>[6x]NSVGQGEFGGAPFKRFLRGTRIVSGGKLKRMTREKAKQVTVAGVPMPRDAEPRHLLVNGATGTGKSVLLRELAYTGLLRGDRMVIVDPNGDMLSKFGRDKDIILNPYDQRTKGWSFFNEIRNDYDWQRYALSVVPRGKTDEAEEWASYGRLLLRETAKKLALIGTPSMRELFHWTTIATFDDLRGFLEGTLAESLFAGSNEASKALTSARFVLSDKLPEHVTMPDGDFSIRSW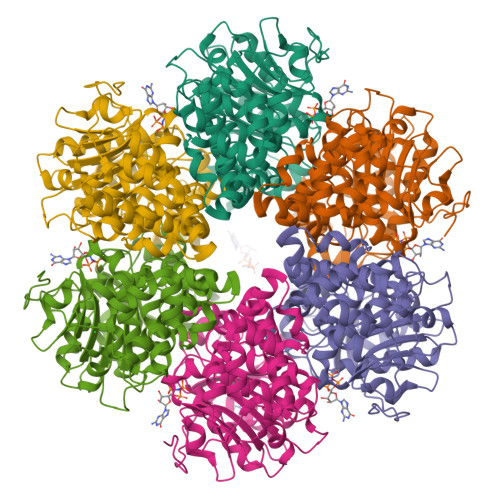LEDPNGGNLFITWREDMGPALRPLISAWVDVVCTSILSLPEEPKRRLWLFIDELASLEKLASLADALTKGRKAGLRVVAGLQSTSQLDDVYGVKEAQTLRASFRSLVVLGGSRTDPKTNEDMSLSLGEHEVERDRYSKNTGKHHSTGRALERVRERVVMPAEIANLPDLTAYVGFAGNRPIAKVPLEIKQFANRQPAFVEGTI> PAGIIPTGNVLSTIEVCAHRCIFDFFKQIRSDDNSLYSAQFDILLGTYCNTLNFVRFLELGLSVACICTKFPELAYVRDGVIQFEVQQPMIARDGPHPVDQPVHNYMVKRIHKRSLSAAFAIASEALSLLSNTYVDGTEIDSSLRIRAIQQMARNLRTVLDSFERGTADQLLGVLLEKAPPLSLLSPINKFQPEGHLNRVARAALLSDLKRRVCADMFFMTRHAREPRLISAYLSDMVSCTQPSVMVSRITHTNTRGRQVDGVLVTTATLKRQLLQGILQIDDTAADVPVTYGEMVLQGTNLVTALVMGKAVRGMDDVARHLLDITDPNTLNIPSIPPQSNSDSTTAGLPVNARVPADLVIVGDKLVFLEALERRVYQATRVAYPLIGNIDITFIMPMGVFQANSMDRYTRHAGDFSTVSEQDPRQFPPQGIFFYNKDGILTQLTLRDAMGTICHSSLLDVEATLVALRQQHLDRQCYFGVYVAEGTEDTLDVQMGRFMETWADMMPHHPHWVNEHLTILQFIAPSNPRLRFELNPAFDFFVAPGDVDLPGPQRPPEAMPTVNATLRIINGNIPVPLCPISFRDCRGTQLGLGRHTMTPATIKAVKDTFEDRAYPTIFYMLEAVIHGNERNFCALLRLLTQCIRGYWEQSHRVAFVNNFHMLMYITTYLGNGELPEVCINIYRDLLQHVRALRQTITDFTIQGEGHNGETSEALNNILTDDTFIAPILWDCDALIYRDEAARDRLPAIRVSGRNGYQALHFVDMAGHNFQRRDNVLIHGRPVRGDTGQAIPITPHHDREWGILSKIYYYIVIPAFSRGSCCTMGVRYDRLYPALQAVIVPEIPADEEAPTTPEDPRHPLHAHQLVPNSLNVYFHNAHLTVDGDALLTLQELMGDMAERTTAILVSSAPDAGAATATTRNMRIYDGALYHGLIMMAYQAYDETIATGTFFYPVPVNPLFACPEHLASLRGMTNARRVLAKMVPPIPPFLGANHHATIRQPVAYHVTHSKSDFNTLTYSLLGGYFKFTPISLTHQLRTGFHPGIAFTVVRQDRFATEQLLYAERASESYFVGQIQVHHHDAIGGVNFTLTQPRAHVDLGVGYTAVCATAALRCPLTDMGNTAQNLFFSRGGVPMLHDNVTESLRRITASGGRLNPTEPLPIFGGLRPATSAGIARGQASVCEFVAMPVSTDLQYFRTACNPRGRASGMLYMGDRDADIEAIMFDHTQSDVAYTD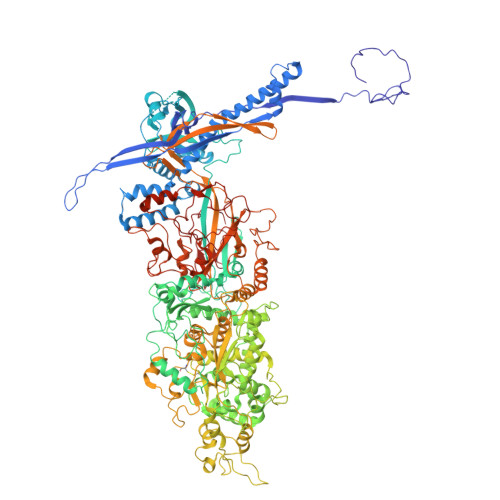RATLNPWASQKHSYGDRLYNGTYNLTGASPIYSPCFKFFTPAEVNTNCNTLDRLLMEAKAVASQSSTDTEYQFKRPPGSTEMTQDPCGLFQEAYPPLCSSDAAMLRTAHAGETGADEVHLAQYLIRDASPLRGCLPL2,4-dioxo-1,2,3,4-tetrahydropyrimidine-5-carbaldehyde 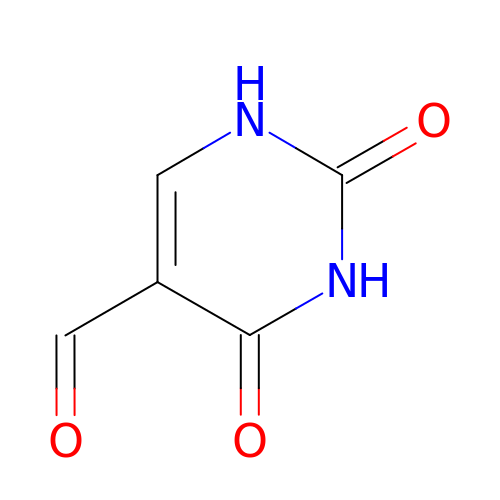| C5 H4 N2 O3 | OHAMXGZMZZWRCA-UHFFFAOYSA-N> GGSMGKTADNHGPVRSETAREGRENQVYSPVTGARLVAGCICLTPDKKQVLMITSSAHKKRWIVPKGGVEKDEPNYETTAQRETWEEAGCIGKIVANLGTVEDMRPPKDWNKDIKQFENSRKDSEVAKHPPRT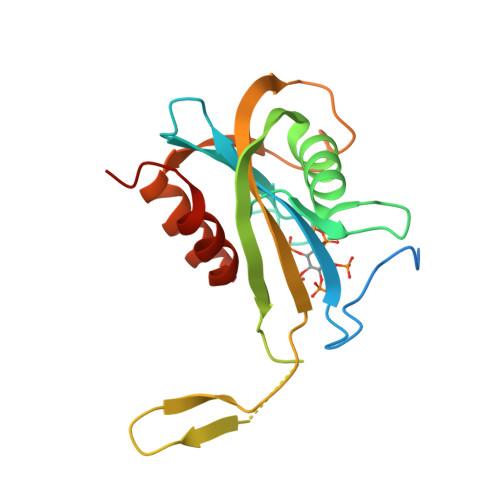EFHFYELEIENLLDKFPECHKRHRKLYSYTEAKQNLIDAKRPELLEALNRSAIIKDDK> VFFSHWTSKYKERNPTEIAYSEDIERIIDSLVTDEITKEEIIHFLFGNFCFHIETMNDQHIADKFKGYQSSCINLKIEPKVDLADLKDHLIQKQQIWESLYGKHLEKIMLRIREKKKKEKEIPDITTAFNQNAAEYEEKYPNCFTNDLSETKTNFSMTWSPSFEKIELSSEVDYNNAIINKFRESFKSSSRVIYNSPYSSINNQTNKARDITNLVRLCLTELSCDTTKMEKQELEDEIDINTGSIKVERTKKSKEWNKQGSCLTRNKNEFCMKETGRENKTIYFKGLAVMNIGMSSKKRILKKEEIKERISKGLEYDTSERQADPNDDYSSIDMSSLTHMKKLIRHDNEDSLSWCERIKDSLFVLHNGDIREEGKITSVYNNYAKNPECLYIQDSVLKTELETCKKINKLCNDLAIYHYSEDMMQFSKGLMVADRYMTKESFKILTTANTSMMLLAFKGDGMNTGGSGVPYIALHIVDEDMSDQFNICYTKEIYSYFRNGSNYIYIMRPQRLNQVRLLSLFKTPSKVPVCFAQFSKKANEMEKWLKNKDIEKVNVFSMTMTVKQILINIVFSSVMIGTVTKLSRMGIFDFMRYAGFLPLSDYSNIKEYIRDKFDPDITNVADIYFVNGIKKLLFRMEDLNLSTNAKPVVVDHENDIIGGITDLNIKCPITGSTLLTLEDLYNNVYLAIYMMPKSLHNHVHNLTSLLNVPAEWELKFRKELGFNIFEDIYPKKAMFDDKDLFSINGALNVKALSDYYLGNIENVGLMRSEIENKEDFLSPCYKISTLKSSKKCSQSNIISTDEIIECLQNAKIQDIENWKGNNLAIIKGLIRTYNEEKNRLVEFFEDNCVNSLYLVEKLKEIINSGSITVGKSVTSKFIRNNHPLTVETYLKTKLYYRNNVTVLKSKKVSEELYDLVKQFHNMMEIDLDSVMNLGKGTEGKKHTFLQMLEFVMSKAKNVTGSVDFLVSVFEKMQRTKTDREIYLMSMKVKMMLYFIEHTFKHVAQSDPSEAISISGDNKIRALSTLSLDTITSYNDILNKNSKKSRLAFLSADQSKWSASDLTYKYVLAIILNPILTTGEASLMIECILMYVKLKKVCIPTDIFLNLRKAQGTFGQNETAIGLLTKGLTTNTYPVSMNWLQGNLNYLSSVYHSCAMKAYHKTLECYKDCDFQTRWIVHSDDNATSLIASGEVDKMLTDFSSSSLPEMLFRSIEAHFKSFCITLNPKKSYASSSEVEFISERIVNGAIIPLYCRHLANCCTESSHISYFDDLMSLSIHVTMLLRKGCPNEVIPFAYGAVQVQALSIYSMLPGEVNDSIRIFKKLGVSLKSNEIPTNMGGWLTSPIEPLSILGPSSNDQIIYYNVIRDFLNKKSLEE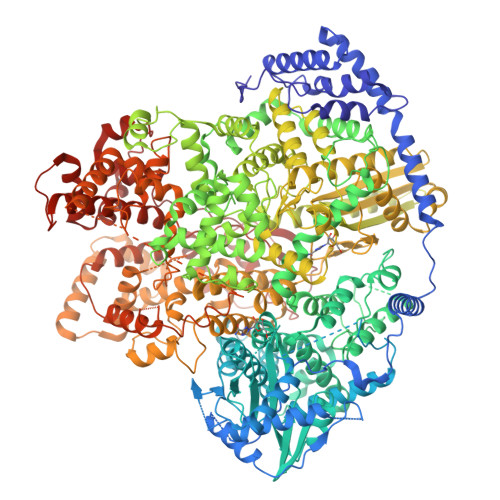VKDSVSSSSYLQMRFRELKGKYEKGTLEEKDKKMIFLINLFEKASVSEDSDVLTIGMKFQTMLTQIIKLPNFINENALNKMSSYKDFSKLYPNLKKNEDLYKSTKNLKIDEDAILEEDELYEKIASSLEMESVHDIMIKNPETILIAPLNDRDFLLSQLFMYTSPSKRNQLSNQSTEKLALDRVLRSKARTFVDISSTVKMTYEENMEKKILEMLKFDLDSYCSFKTCVNLVIKDVNFSMLIPILDSAYPCESRKRDNYNFRWFQTEKWIPVVEGSPGLVVMHAVYGSNYIENLGLKNIPLTDDSINVLTSTFGTGLIMEDVKSLVKGKDSFETEAFSNSNECQRLVKACNYMIAAQNRLLAINTCFTRKSFPFYSKFNLGRGFISNTLALLSTIYSKEES> GPGSMAPLPRKALLAITSAHPPFWPDGKRTGLFFSEALHPFNELTAAGFEVDVASETGTFGWDEHSLTQEYLSKEDEKVLHSEHNHFMEKMNKQVFKAGDLAPHDYGLMFVCGGHGALYDFPHAKHLQNIAQDIYKRGGVIG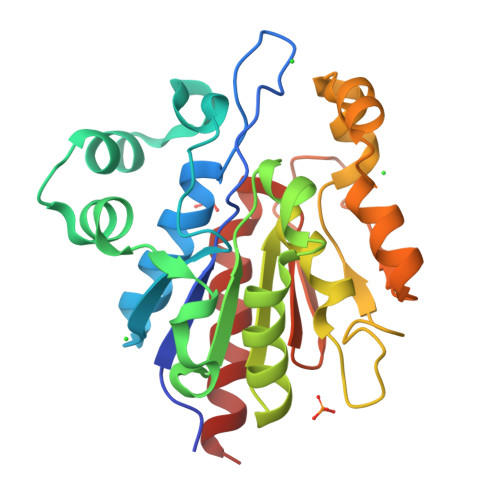AVCHGPAMLPGIHDENGDSVIKDKTVTGFTTKGEIMIKVIDKMREDHLHTIADMAQTANAEYVPPEDPWDDFCKVDGRIVTGANPQSATNTARDTIKVYEGIVNE>[2x]TSGVLLESQTKITDGALHFDGKKLNHNTFENPSKSQAYDYFFGRNISAHGDAVKPYKHFVFMTWYKGGKEERNVMLSRFNTKTGVVKTIQFPHRHTGFRGDPLVGESHNTI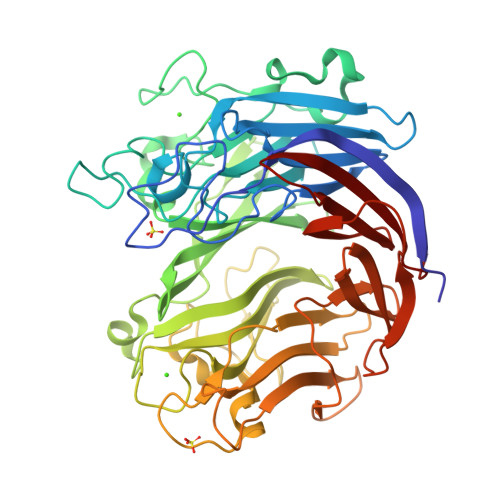GLAVSPLNGTIHMVYDMHAYVDDDETGRFKGRFVDDFFRYSFSVAGAADVPDDEFTLEQFVKDTSELSQGADDYKHLTMTGNLQDKENFSALTYPKFYTSDDGELLHYMRWGGNNNGAYYFNKYDAKNQKWTRFTPFNHKDQKTHGNAYNWGLYGQMKYINGKLRVGFQQRSANNDDRFKYQNGVYYAYSDHPDGLGNWKNVDGEDMTWPLVNSDEIKIFEPGDYIDHTAPNSVHIVTGFDWTVTENDDVHFITHVRSTDTKRSDYKEVSIHAFKPANAVDFTITTDFTGADSIYTSGDSIFIIGLKNGYPFVEKAKGGSNDFEVVYQQASGVKFDHGTIHIENGKAYYYLMEKGAGNALPLHLQVIDLGVT>[4x]GSHMEVTTTAYKDQKPGTSGLRKKVTVFQQPNYTANFVQSTFNALHRQGAVPDVLVVGGDGRYYTSEAVQVILKVSAANGVRCVWVGQHGLLSTPAVSTMVRRRRDADGRKATGAFILTASHNPGGPDADFGIKYNSENGGPAPEKLTSQIYEETVKITHIKMAPTLPEVDIHTLGTYTFDDYNFQVEV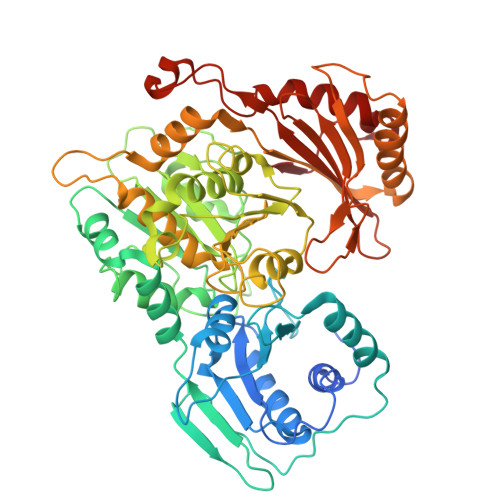VDSLADYAAYMQEVFDFEAIRALVQRLDFKVHVDSLHGVSGPYVDRIFHEGLGVPKTSLFRTNVLPDFGGCHPDPNLTYAADLVHVMGLLPDGNANPAMKHISTVPSFGVAFDGDADRNMILGCRFFVNPSDSLAVLAANADCVPFFTQSSSSGLKAVARSMPTSGAVDRVAAAHDFALFEVPTGWKFFGNLMDSKDLYGGKDFNPLLCGEESFGTGSNHIREKDGIWASLFWLSVIAKRNAPGTPLVGVQQIVEEHWATYGRNYYSRYDYEDVSAEAAKAVMDTVENTVVDDVPNLNGVACKTIDNFSYTDPIDGSVSTKQGVRVLFEDGSRFVLRLSGTGSSGATIRLYLEQYMDSATVKSHLAEKTLPTASTALKALIGVALQVSKMESLTGRKTPTVIT> SNARIMEEKALEVYDLIRTIRDPEKPN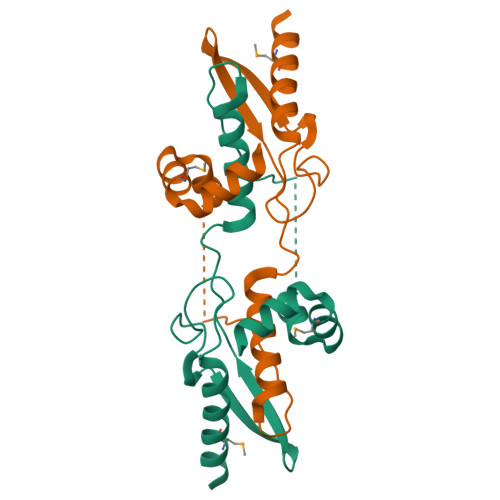TLEELEVVSESCVEVQEINEEEYLVIIRFTPTVPHCSLATLIGLCLRVKLQRCLPFKHKLEIYISEGTHSTEEDINKQINDKERVAAAMENPNLREIVEQCVL> GSMAQILPIRFQEHLQLQNLGINPANIGFSTLTMESDKFICIREKVGEQAQVVIIDMNDPSNPIRRPISADSAIMNPASKVIALKAGKTLQIFNIEMKSKMKAHTMTDD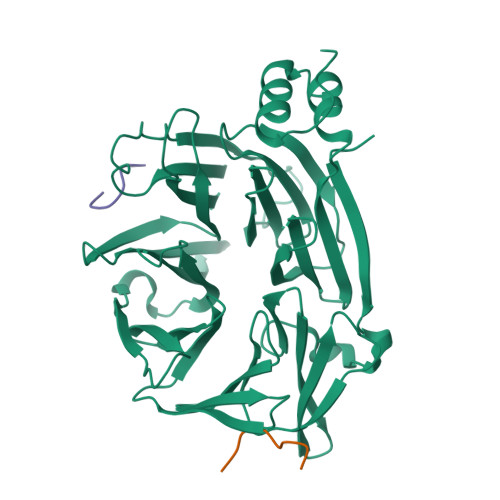VTFWKWISLNTVALVTDNAVYHWSMEGESQPVKMFDRHSSLAGCQIINYRTDAKQKWLLLTGISAQQNRVVGAMQLYSVDRKVSQPIEGHAASFAQFKMEGNAEESTLFCFAVRGQAGGKLHIIEVGTPPTGNQPFPKKAVDVFFPPEAQNDFPVAMQISEKHDVVFLITKYGYIHLYDLETGTCIYMNRISGETIFVTAPHEATAGIIGVNRKGQVLSVCVEEENIIPYITNVLQNPDLALRMAVRNNLAGAEEL;>[2x]CGDLLNLDLG> LFLLTVC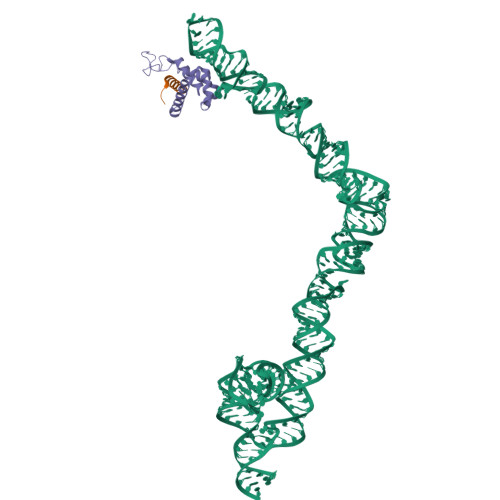TTVLVSGWVVLGWME;> TLDDFLEQLGQVRNMGPLDELLQMMPGAGKMKGLKNIQVDEKQLNHVEAIIKSMTVLEKEQPDIINASRRKRIAKGSGTSVQEVNRLLKQFDEMKKMMKQMT> MTVKISHTADIQAFFNQVAGLDHAEGKPRFKQIILRVLQDTARLIEDLEITEDEFWHAVDYLNRLGGRNEAGLLAAGLGIEHFLDLLQDAKDAEAGLGGGTPRTIEGPLYVAGAPLAQGEVRMDDGTDPGVVMFLQGQVFDANGKPLAGATVDLWHANTQGTYSYFDSTQSEFNLRRRIITDAEGRYRARSIVPSGYGCDPQGPTQECLDLLGRHGQRPAHVHFFISAFGHRHLTTQINFAGDKYLWDDFAYATRDGLIGELRFVEDAAAARDRGVQGE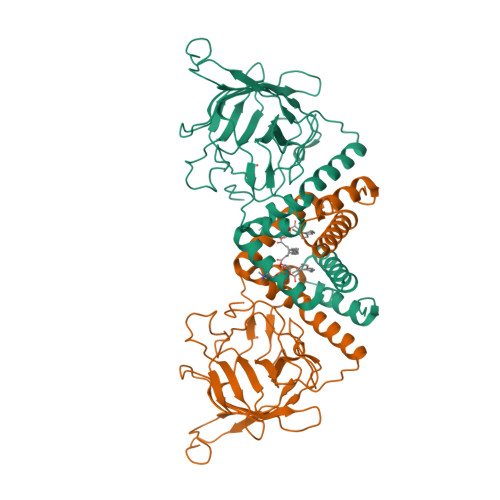RFAELSFDFRLQGAQSPDAEARSHRPRALQEG> MKTWPAPTAPTPVRATVTVPGSKSQTNRALVLAALAAAQGRGASTISGALRSRDTELMLDALQTLGLRVDGVGSELTVSGRIEPGPGARVDCGLAGTVLRFVPPLAALGSVPVTFDGDQQARGRPIAPLLDALRELGVAVDGTGLPFRVRGNGSLAGGTVAIDASASSQFVSGLLLSAASFTDGLTVQHTGSSLPSAPHIAMTAAMLRQAGVDIDDSTPNRWQVRPGPVAARRWDIEPDLTNAVAFLSAAVVSGGTVRITGWPRVSVQPADHILAILRQLNAVVIHADSSLEVRGPTGYDGF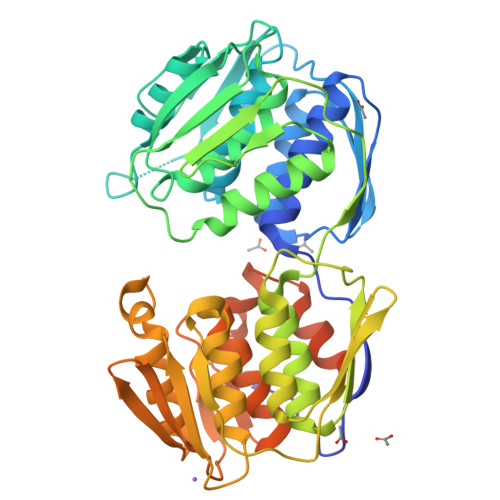DVDLRAVGELTPSVAALAALASPGSVSRLSGIAHLRGHETDRLAALSTEINRLGGTCRETPDGLVITATPLRPGIWRAYADHRMAMAGAIIGLRVAGVEVDDIAATTKTLPEFPRLWAEMVGPGQGWGYPQPRSGQRARRATGQGSGGKLAAALEHHHHH>[4x]MKAHPKEMVPLMGKRVAAPSGNPAVLPEKRPAEITPTKKSAHFFLEIEGFEPNPTVAKTSPPVFSKPMDSNIRQCISGNCDDMDSPQSPQDDVTETPSNPNSPSAQLAKEEQRRKKRRLK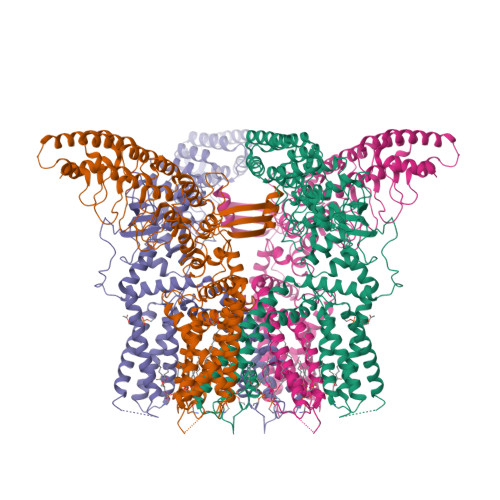KRIFAAVSEGCVEELVELLVELQELCRRRHDEDVPDFLMHKLTASDTGATCLMKALLNINPNTKEIVRILLAFAEENDILGRFINAEYTEEAYEGQTALNIAIERRQGDIAALLIAAGADVNAHAKGAFFNPKYQHEGFYFGETPLALAACTNQPEIVQLLMEHEQTDITSRDSRGNNILHALVTVAEDFKTQNDFVKRMYDMILLRSGNWELETTRNNDGLTPLQLAAKMGKAEILKYILSREIKEKRLRSLSRKFTDWAYGPVSSSLYDLTNVDTTTDNSVLEITVYNTNIDNRHEMLTLEPLHTLLHMKWKKFAKHMFFLSFCFYFFYNITLTLVSYYRPREEEAIPHPLALTHKMGWLQLLGRMFVLIWAMCISVKEGIAIFLLRPSDLQSILSDAWFHFVFFIQAVLVILSVFLYLFAYKEYLACLVLAMALGWANMLYYTRGFQSMGMYSVMIQKVILHDVLKFLFVYIVFLLGFGVALASLIEKCPKDNKDCSSYGSFSDAVLELFKLTIGLGDLNIQQNSKYPILFLFLLITYVILTFVLLLNMLIALMGETVENVSKESERIWRLQRARTILEFEKMLPEWLRSRFRMGELCKVAEDDFRLCLRINEVKWTEWKTHVSFLNEDPGPVRRTDFNKIQDSSRNNSKTTLNAFEEVEEFPETSV THYMIDINE-5'-(DITHIO)PHOSPHATE | C10 H15 N2 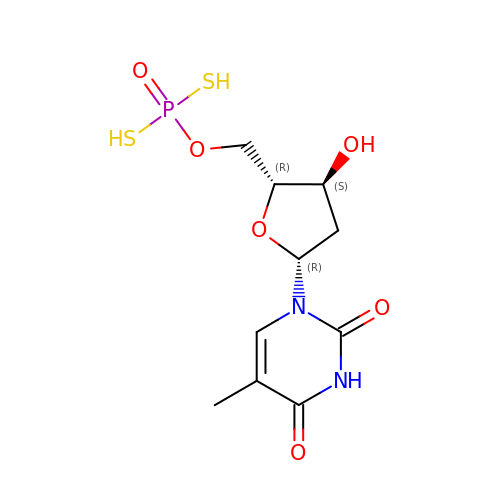O6 P S2 | KMPXQZWMYQHTNT-XLPZGREQSA-N(2E)-3-{5-[(2,4-diaminopyrimidin-5-yl)methyl]-2,3-dimethoxyphenyl}-1-[(1R)-1-(2-methylpropyl)phthalazin-2(1H)-yl]prop-2-en-1-one 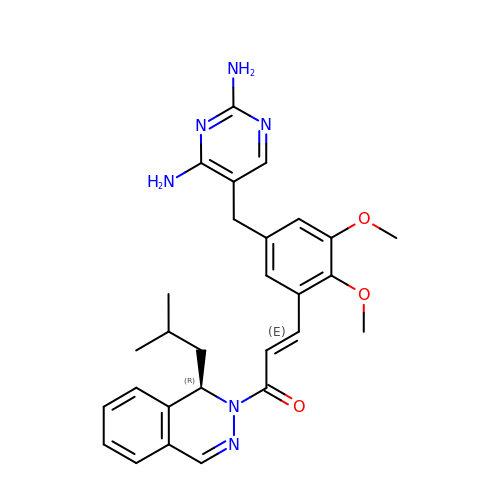| C28 H32 N6 O3 | ZISYTWICFLBNJQ-JJNABOQBSA-N3-methyl-8-[(piperidin-4-yl)amino]-1,2-dihydro-1,7-naphthyridin-2-one 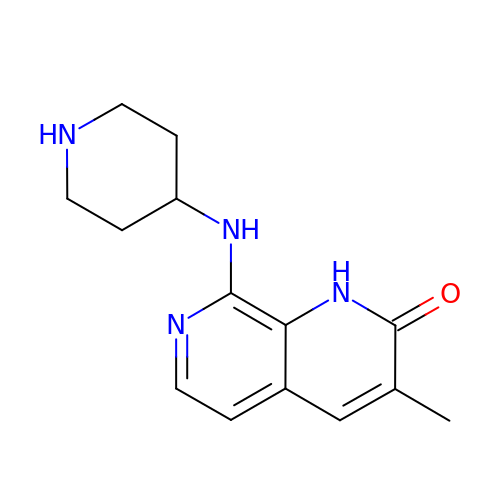| C14 H18 N4 O | WPUMQOWFWIAZCU-UHFFFAOYSA-N Phosphotriesterase-like Lactonases (PLLs) are appealing candidates, being natural lactonases endowed with promiscuous phosphotriesterase activity. PTEs and PLLs belong to the amidohydrolase superfamily, and share the same (β/α)8 barrel topology. SsoPox exhibits high acyl-homoserine lactones and oxo-lactones hydrolysis abilities, and promiscuous, low phosphotriesterase activity. SsoPox is a very appealing candidate for the bioremediation of phosphotriesters because of its unique thermal stability, and its ability to resist aging, solvent and protease treatments.

Of them, the most active variants, αsA1 (C258L-I261F-W263A), αsA6 (F46L-C258A-W263M-I280T), αsB5 (V27A-I76T-Y97W-Y99F-L130P-L226V), αsC6 (L72I-Y99F-I122L-L228M-F229S-W263L), and αsD6 (V27A-Y97W-L228M-W263M) were subject to kinetic and structural characterization. It should be noted that αsA1 was obtained in a previous engineering effort, and that four of the five selected variants contained a substitution of the key residue W263. Overall, all variant exhibits improved catalytic efficiencies against all tested substrates, with the exception of αsA1 with malathion (~2-fold decrease). Interestingly, variants αsA6 and αsC6 exhibit enhanced lactonase activity against γ- and δ-lactones, while αsA1, αsB5 and αsD6 show reduced lactonase catalytic efficiencies. Although the active sites of the improved variant structures superpose well onto the wt-structure, all selected mutants display altered loop 8 conformations. Changes are subtle for some of the variants (e.g. αsA1), but are large for others (e.g. αsC6). Because part of loop 8, including position 263, is located at the enzyme dimer interface, altered loop 8 conformations modulate the relative orientation of both monomers. In the case of the mutants characterized in this study, the dimer reorientation yields significant displacement up to 5.2 Å (e.g., αsA1, between equivalent carbon α positions), as compared to wt-SsoPox.

>MRIPLVGKDSIESKDIGFTLIHEHLRVFSEAVRQQWPHLYNEDEEFRNAVNEVKRAMQFGVKTIVDPTVMGLGRDIRFMEKVVKATGINLVAGTGIYIYIDLPFYFLNRSIDEIADLFIHDIKEGIQGTLNKAGFVKIAADEPGITKDVEKVIRAAAIANKETKVPIITHSNAHNNTGLEQQRILTEEGVDPGKILIGHLGDTDNIDYIKKIADKGSFIGLDRYGLDLFLPVDKRNETTLRLIKDGYSDKIMISHDYLCTFDAGTAKPEYKPKLAPRWSITLIFEDTIPFLKRNGVNEEVIATIFKENPKKFFS[4x]> SPSVEACGYSDRIIQITRGDSTITSQDVANAVVGYGVWPHYLTPQDATAIDKPTQPDTSSNRFYTLDSKMWNSTSKGWWWKLPDALKDMGIFGENMFYHFLGRSGYTVHVQCNASKFHQGTLLVVMIPEHQLAT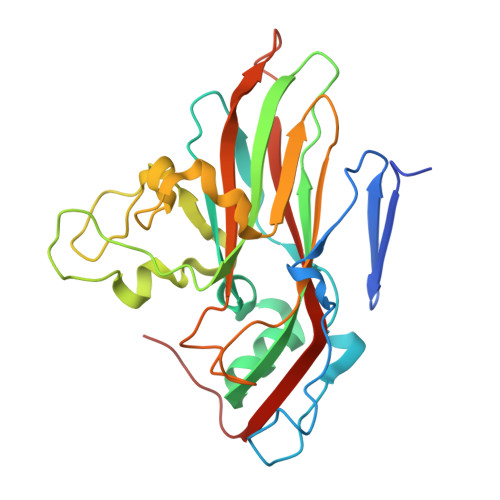VNKGNVNAGYKYTHPGEAGREVGTQVENEKQPSDDNWLNFDGTLLGNLLIFPHQFINLRSNNSATLIVPYVNAVPMDSMVRHNNWSLVIIPVCQLQSNNISNIVPITVSISPMCAEFSGARAKTVVQ> GLPVYVTPGSGQFMTTDDMQSPCALPWYHPTKEIFIPGEVKNLIEMCQVDTLIPINSTQSNIGNVSMYTVTLSPQTKLAEEIFAIKVDIASHPLATTLIGEIASYFTHWTGSLRFSFMFCGTANTTLKVLLAYTPPGIGKPRSRKEAMLGTHVVWDVGLQSTVSLVVPWISASQYRFTTPDTYSSAGYITCWYQTNFVVPPNTPNTAEMLCFVSGCKDF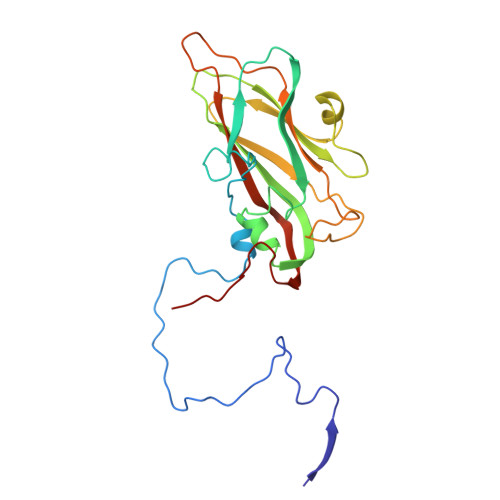CLRMARDTDLHKQTGPITQ>MTRPEQPRPESADLPAPTLEVIPLGGMGEIGKNITVFRYGDEIVVVDGGLAFPKAHQMGIDLIVPRIDYLLEHQDKIKGWILTHGHEDHIGGLPYIFARLPRVPVYGLPLTLALVREKLSEFGLQDVDLREVTYGDEVRFGQSFVAEFFCMTHSIPDNAGYILKTPVGDVLHTGDFKIDPDVGTGAGIVSDLERVEQAGKDGVLLLISDSTNAERPGHTPSEAEIARNLEEIIKGCRGRVFLTTFASQVYRIQNILDLAHRQGRRVVMEGRSMIKYAQAAQATGHMNPPEPFLTSEEVGELQDQQVLFVCTGSQGQPMAVLGRLAFGTHAKIALRRGDTVILSS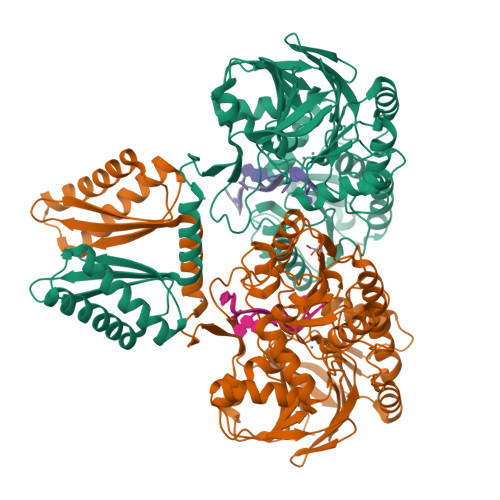NPIPGNEDAVNLIVNRLYEIGVDVVYPPTYRVHASGHASQEELATILNLTRPKFFLPWHGEPRHQINHAKLAQTLPRPPKRTLIAKNGDIVNLGPDEFRVSGTVAAGAVYVDGLGVGDVNDDVLLDRVNLSQEGLLILTAVLHPTPHVEVVARGFARPNRDLELQIRRVALEAVEQGLREKKRLEDVRDDMYGAVRRFTRKATGRNPVLIPMIVD[2x]>SRAYDLVVIGAGSGGLEAGWNAASLHKKRVAVIDLQKHHGPPHYAALGGTCVNVGCVPKKLMVTGANYMDTIRESAGFGWELDRESVRPNWKALIAAKNKAVSGINDSYEGMFADTEGLTFHQGFGALQDNHTVLVRESADPNSAVLETLDTEYILLATGSWPQHLGIEGDDLCITSNEAFYLDEAPKRALCVGGGYISIEFAGIFNAYKARGGQVDLAYRGDMILRGFDSELRKQLTEQLRANGINVRTHENPAKVTKNADGTRHVVFESGAEADYDVVMLAIGRVPRSQTLQLEKAGVEVAKNGAIKVDAYSKTNVDNIYAIGDVTDRVMLTPVAINEGAAFVDTVFANKPRATDHTKVACAVFSIPPMGVCGY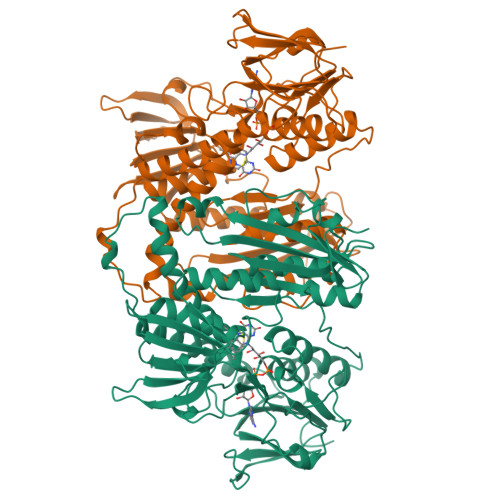VEEDAAKKYDQVAVYESSFTPLMHNISGSTYKKFMVRIVTNHADGEVLGVHMLGDSSPEIIQSVAICLKMGAKISDFYNTIGVHPTSAEELCSMRTPAYFYEKGKRVEKIDSNL[2x]>[2x]MSSAPRRPAKGADSFCTPEPESLGPGTPGFPEQEEDELHRTLGVERFEEILQEAGSRGGEEPGRSYGEEDFEYHRQSSHHIHHPLSTHLPPDARRRKTPQGPGRKPRRRPGASPTGETPTIEEGEEDEDEASEAEGARALTQPSPVSTPSSVQFFLQEDDSADRKAERTSPSSPAPLPHQEATPRASKGAQAGTQVEEAEAEAVAVASGTAGGDDGGASGRPLPKAQPGHRSYNLQERRRIGSMTGAEQALLPRVPTDEIEAQTLATADLDLMKSHRFEDVPGVRRHLVRKNAKGSTQSGREGREPGPTPRARPRAPHKPHEVFVELNELLLDKNQEPQWRETARWIKFEEDVEEETERWGKPHVASLSFRSLLELRRTLAHGAVLLDLDQQTLPGVAHQVVEQMVISDQIKAEDRANVLRALLLKHSHPSDEKDFSFPRNISAGSLGSLLGHHHGQGAESDPHVTEPLMGGVPETRLEVERERELPPPAPPAGITRSKSKHELKLLEKIPENAEATVVLVGCVEFLSRPTMAFVRLREAVELDAVLEVPVPVRFLFLLLGPSSANMDYHEIGRSISTLMSDKQFHEAAYLADEREDLLTAINAFLDCSVVLPPSEVQGEELLRSVAHFQRQMLKKREEQGRLLPTGAGLEPKSAQDKALLQMVEAAGAAEDDPLRRTGRPFGGLIRDVRRRYPHYLSDFRDALDPQCLAAVIFIYFAALSPAITFGGLLGEKTQDLIGVSELIMSTALQGVVFCLLGAQPLLVIGFSGPLLVFEEAFFSFCSSNHLEYLVGRVWIGFW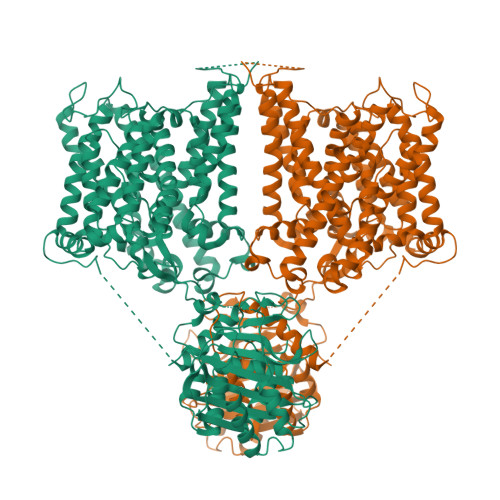LVFLALLMVALEGSFLVRFVSRFTQEIFAFLISLIFIYETFYKLVKIFQEHPLHGCSASNSSEVDGGENMTWAGARPTLGPGNRSLAGQSGQGKPRGQPNTALLSLVLMAGTFFIAFFLRKFKNSRFFPGRIARVIGDFGVPIAILIMVLVDYSIEDTYTQKLSVPSGFSVTAPEKRGWVINPLGEKSPFPVWMMVASLLPAILVFILIFMETQITTLIISKKERMLQKGSGFHLDLLLIVAMGGICALFGLPWLAAATVRSVTHANALTVMSKAVAPGDKPKIQEVKEQRVTGLLVALLVGLSIVIGDLLRQIPLAVLFGIFLYMGVTSLNGIQFYERLHLLLMPPAAHPDVTYVKKVRTLRMHLFTALQLLCLALLWAVMSTAASLAFPFILILTVPLRMVVLTRIFTDREMKCLDANEAEPVFDEREGVDEYNEMPMPV>ADQVDPQLKFAMQRDLGIFPTQLPQYLQTEKLARTQAAAIEREFGAQFAGSWIERNEDGSFKLVAATSGARKSSTLGGVEVRNVRYSLKQLQSAMEQLDAGANARVKGVSKPLDGVQSWYVDPRSNAVVVK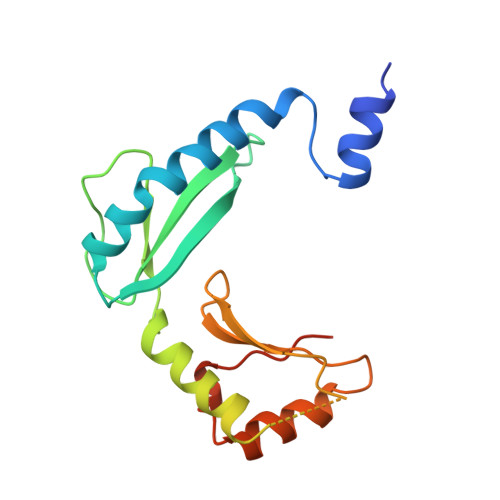VDDGATDAGVDFVALSGADSAQVRIESSPGKLQTT[3x]> MVENNYLSVSEKTELEIAKQKLKNSKDPAEREKAQQKYDALLE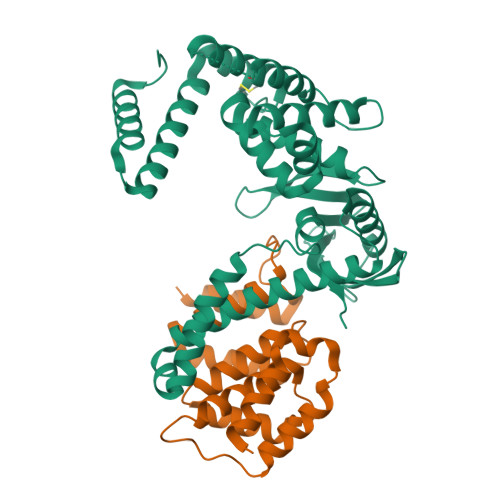KDISSDKAVITACSNGQAASAACAGERLKVIAAKGGYETGHYNNQVSDMYPDAYGQIVNLLNITSVDAQNQQQVKDAMVNYAMVQFGVDRATAQAYVETYDGMKVVAASMAPVIGAAAASKIEVLAGKQRLSNSFEVSSLPDANGKNHITAVKGDAKIPVDKIELYMRGKASGDLDSLQAEYNSLKDARISSQKEFAKDPNNAKRMEVLEKQIHNIERSQDMARVLEQAGIVNTASNNSMIMDKLLDSAQGATSANRKTSVVVSGPNGNVRIYATWTILPDGTKRLSTVNTGTFK;> MINVNSTAKDIEGLESYLANGYVEANSFNDPEDDALECLSNLLVKDSRGGLSFCKKILNSNNIDGVFIKGSALNFLLLSEQWSYAFEYLTSNADNITLAELEKALFYFYCAKNETDPYPVPEGLFKKLMKRYEELKNDPDAKFYHLHETYDDFSKAYPLNNHHHHHH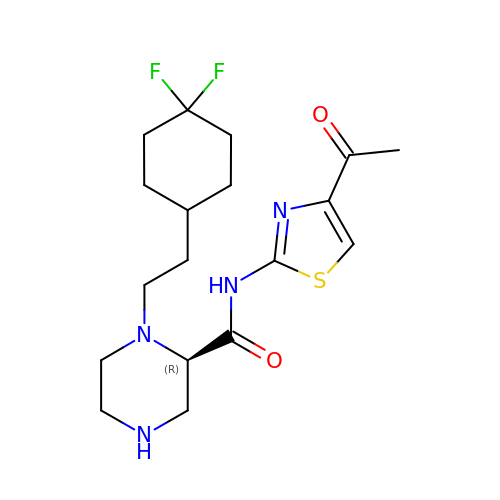(2~{R})-1-[2-[4,4-bis(fluoranyl)cyclohexyl]ethyl]-~{N}-(4-ethanoyl-1,3-thiazol-2-yl)piperazine-2-carboxamide | C18 H26 F2 N4 O2 S | XAAULFWATXYIOV-OAHLLOKOSA-N>SNATVFLSGSA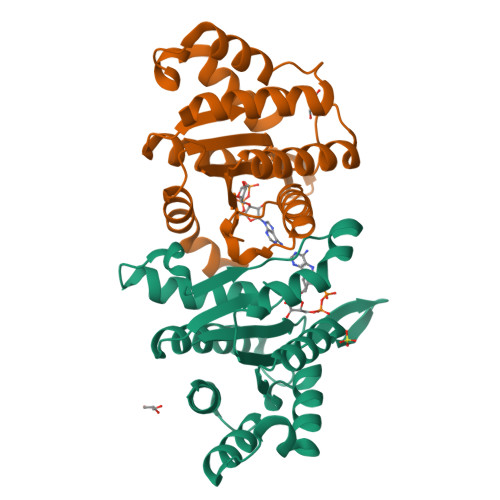VEYNHWETEHAEQFIHQLSKELIRKDFNIVSGFGLGVGSFVINGVLEELYMNQGTIDDDRLILRPFPQGKKGEEQWDKYRRDMITRTGVSIFLYGNKIDKGQVVKAKGVQSEFNISFEQNNYVVPVGATGYIAKDLWNKVNEEFETYYPGADARMKKLFGELNNEALSIEELINTIIEFVEILSN[2x]>SNAMADEIAKAQVARPGGDTIFGKIIRKEIPAKIIFEDDRCLAFHDISPQAPT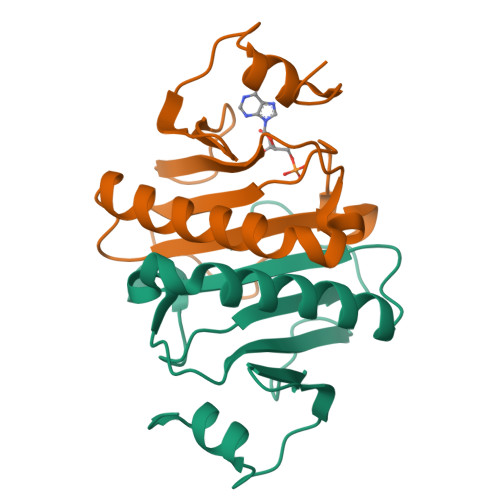HFLVIPKKHISQISVAEDDDESLLGHLMIVGKKCAADLGLNKGYRMVVNEGSDGGQSVYHVHLHVLGGRQMHWPPG[4x]>[2x]AMALTGCSEKININEDKISHKIDIPDSAWTIGIGEKFKNAGHPNVKYPMIDDSYVQGAPLGGFGAGTIGRTYNGGFSRW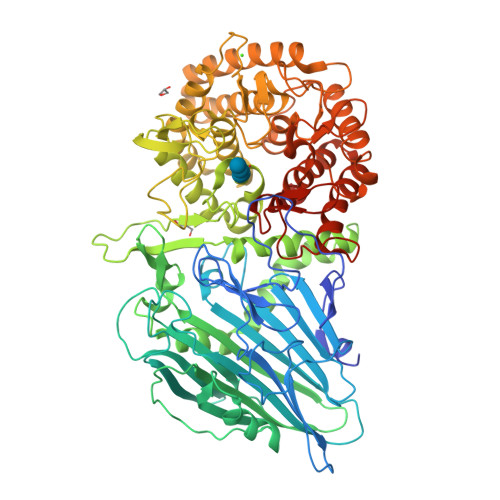HLEIGKNKYTTVYANQFSVFQKVEGNKDGVAQVLYAGEPENGYLSSWKWDYPKESGMYYALYPNSWYTYTNKDLPVQLAVKQFSPIIPYNYKETSYPVAVFKWTAYNPTNKNVDVSIMFTWQNMIGFFGKQVNVNSGNFNKIIKDKSKDSEIVAAVMGNISNDNEEWNGEYSIGVKKVPGVDISYKAKFVTTGDGSDLWHEFSKNGILDNKDDETPTKQDGIGSAIAVNFKLQPGQTIEVPFALSWDLPIMKFGGGDKWYKMYTKYFGKNGKNSFAILKEALNNYQKWEKMIDDWQKPILSNKSKPDWYKTALFNELYYLADGGTAWENGKVGEKDKRTNNMFGLLGCFDYNYYETLDVRFYGSFPLVMLWPDIEKQVMRQFADTINVQDSSEFKVGSNGAMAVKKVQGMIPHDLGSSYALPWIKINAYDWQNPNIWKDLNSKYVLLVYRDYVLTGKTDKEFLKYTWKSVKTALDKLKEMDKDNDGIPDNEGIPDQTYDTWSMKGTSAYCGSLWLAALKAAQEIGKVLKDNEAYIKYNEWYKIAQQNFEKELWNGEYYNFDTESDHKDSIMADQLAGQWYADILRLGDILPKDHVQKALKKIYEFNVMKFENGKMGAVNGMRPDGIVDESDIQAQEVWTGVTYALASFMKYRGMTEEAYNTAYGVYKMTYDKSGKGYWFRTPEAWTKDGNYRASMYMRPLSIWSMEVNYNEVLEHHHHHH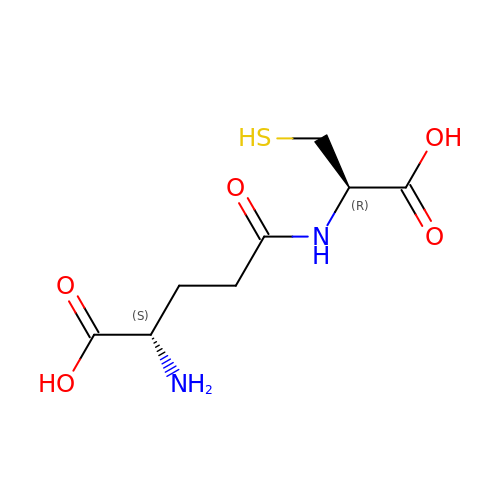GAMMA-GLUTAMYLCYSTEINE | C8 H14 N2 O5 S | RITKHVBHSGLULN-WHFBIAKZSA-N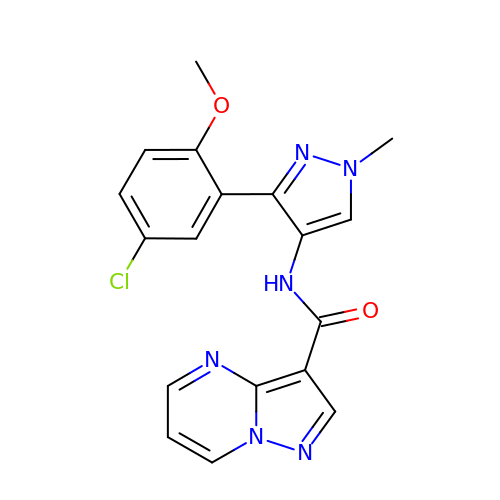N-[3-(5-chloro-2-methoxyphenyl)-1-methyl-1H-pyrazol-4-yl]pyrazolo[1,5-a]pyrimidine-3-carboxamide | C18 H15 Cl N6 O2 | PBBLZBUJHLNSRL-UHFFFAOYSA-N> YTRKMWSVQESEWLKQGVVRYGVGHWERIRSAFPFAGRTAVNLK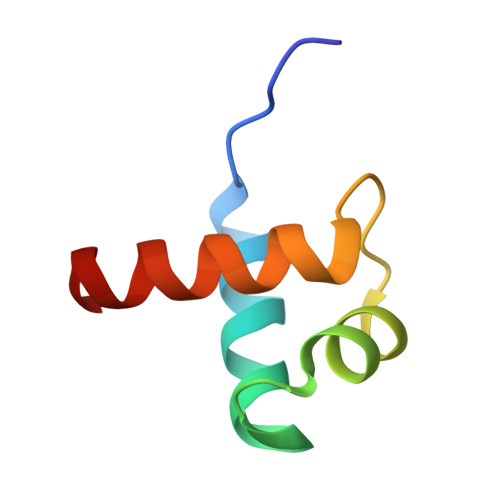DRWRTMVKLKM The structure-specific nuclease, flap endonuclease-1 (FEN1) plays a vital role in maintaining genome integrity by precisely processing intermediates of Okazaki fragment maturation, long-patch excision repair, telomere maintenance, and stalled replication forks. FEN1 preferentially binds to double flap substrates with a one nt 3′-flap and any length of 5′-flap, including zero. It catalyses a single hydrolytic incision one nucleotide (nt) into dsDNA to yield nicked DNA ready for direct ligation. Here crystallographic analyses uncover an unprecedented electrostatic steering of an inverted 5′-flap through the human FEN1 (hFEN1) helical gateway.

To obtain structures of hFEN1 with a ss 5′-flap substrate for insight into ss 5′-flap selection, we crystallized three hFEN1 active site mutants D86N, R100A and D233N with a double-flap (DF) substrate and with Sm3+. In the hFEN1-D86N and hFEN1-R100A structures, the ssDNA (5′-flap) region of the substrate threaded through the tunnel formed by the gateway/cap. In both threaded substrate structures, the ss 5′-flap phosphodiester backbone is ‘inverted’ between the +1 and +2 positions, with the +2 and +3 phosphates facing away from the active site metals and the DNA bases facing the metals. The overall inverted flap orientation resembles the hFEN1-R100A structure with the +1 phosphate remaining within 7 Å of Arg104, but shifted towards Arg103, presumably due to Arg100 removal. In the hFEN1-R100A structure, the scissile phosphodiester bond was ∼4–5 Å away from the metal ions, although −1 and +1 nts have moved towards the active site and away from the template strand. The −1 and −2 nts display less base overlap (stacking), and the +1 and −1 nts are no longer hydrogen bonded to the template strand (4–6 Å apart). Notably, as duplex DNA is not shifted close to the catalytic metal in the R100A structure, this structure may represent a pre-reactive substrate form. Its Tyr40 stacks at a 50° angle with the +1 nt and resembles the other hFEN1 structures, suggesting that the Tyr40 rotamer is linked to shifting duplex DNA into a catalytic position. On the basis of the hFEN1-R100A structure, Arg100 is also likely essential for shifting of the scissile phosphate into direct contact with the catalytic metals. On the basis of the hFEN1-R100A structure, we mutated three basic residues (Arg103, Arg104 and Lys132) positioned to guide the phosphodiester backbone and stabilize the inverted ssDNA orientation.

> GIQGLAKLIADVAPSAIRENDIKSYFGRKVAIDASMSIYQFLIAVRQGGDVLQNEEGETTSHLMGMFYRTIRMMENGIKPVYVFDGKPPQLKSGELAKASERRAEAEKQLQQAQAAGAEQEVEKFTKRLVKVTKQHNDECKHLLSLMGIPYLDAPSEAEASCAALVKAGKVYAAATEDMDCLTFGSPVLMRHLTASEAKKLPIQEFHLSRILQELGLNQEQFVDLCILLGSDYCESIRGIGPKRAVDLIQKHKSIEEIVRRLDPNKYPVPENWLHKEAHQLFLEPEVLDPESVELKWSEPNEEELIKFMCGEKQFSEERIRSGVKRLSKSRQGSTLEVLFQ> GPLGSYGDAIPEVKAILEAKNEEELVTFTSRWSAEERKELRTQFQDTTGLEFIAFLKKCIKNGPYEDVMALGWDCNISARVNVIKKAMKNVNDFRAIHDVVLIATPDERLKLAQAYKEKTGNDLLQDFVDQIPLTSAASYLCHLAIRENRTPRGSVASDAEVLKHNLIDADEPDHEAVVRLIITSTADEYKEINHR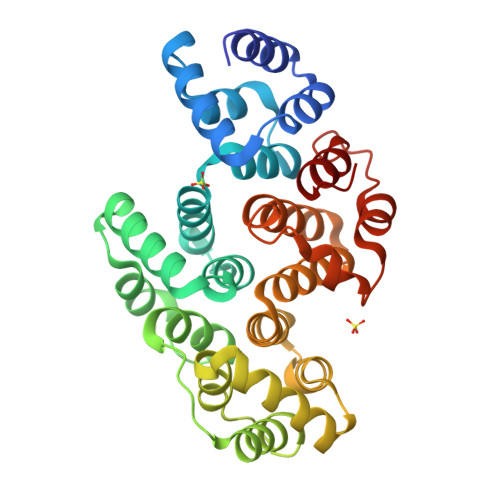FEVLTGKSVQEAIETRYADKENARGLCIAHYYNLAPARAVAYAFHSAVETQNDDMAYEQAARITGLFHDLHKFAWVHYACWGVMRDDILSRFQSKEANKVNFRDACLMFWKLAK Altogether CD38 appears to be a key player in the biosynthesis of calcium messengers which are involved in a wide range of cellular functions. Thus, the catalytic transformation of NAD+ involves the formation, via a ribooxocarbenium ion-like transition state, of a unique reaction intermediate that partitions between several competing pathways such as an irreversible hydrolytic process leading to ADP-ribose and a reversible minor pathway that governs the formation of cADPR. The L-shaped structure of bCD38 consists of two distinct domains separated by a cleft and connected by a hinge region. α-Helices are found mainly in the N-terminal and membrane-proximal domain of this transmembrane protein, whereas β-sheets are preponderant in the distal C-terminal domain. The active site of bCD38 consists in a funnel-shaped cavity with a fairly rigid structure; it buries the NMN+ moiety of the substrate and its scissile bond in its deepest non-polar and least solvent accessible region, whereas the AMP moiety interacts with its more solvent-exposed region, at the entrance of the catalytic cleft.

Superposition of the E218Q mutant on the wt apo enzyme showed no differences between the structures (not shown) demonstrating the conservative nature of the mutation. This suggests that the active site geometry is maintained in the mutant and that the kinetic effects of the mutation (see below) are due to an intrinsic catalytic function of Glu218 side chain. Similarly, in the E218Q mutant, both Oε1 and Nε2 atoms of the amide group of Gln218 are interacting with water molecules and the Nε2 is at a distance of 2.9–3.0 Å from the oxygen atom of Ser185 side chain. Soaking crystals of the catalytically impaired E218Q mutant of bCD38 with NAD+ failed to capture uncleaved substrate or any of the reaction products, nicotinamide and ADP-ribose. Altogether our results indicate that the E218Q mutant still carries a measurable residual catalytic activity. Finally, the stabilization of the oxocarbenium ion intermediate by Glu218 can occur either by charge-charge stabilization or via a collapse to form a covalent acylal bond at its C1′-position. Importantly, such non-polar microenvironment-related effects could explain the residual catalytic activity of Glu218 mutants of bCD38 such as E218Q (see above).

>YKWHYSGLNRWHGAGSTADFQKIIQERCDTYTQTIRPGSRSRNCQAIRQAFMSAFISKDPCKATKEDYNSLINLAPPTVPCGQQVFWSKTKELAHEYAKRRRLMTLEDTLLGYLADGLRWCGEPGSSDLNIWSCPDWRKDCRTNYLSVFWEVLSERFAESACNTVRVVLNGSLENAFDSMSIFGRVQAPNLRPQVELEAWLVHDTGKPPSDSCSGSSIRKLKSILDGRNVKFRCMDNLSRDQFLQRS[2x]>[4x]KRKIIFLSSPYGFSQQQKTLLLPPIVRALEALGIEVWEPFARNNQIDFSQADWAYRVAQADLQDVKNCDGIFAVVNGTPPDEGVMVELGMAIALNKAIFLFRDDFRRCSDNERYPLNLMLFAGLPEIGWENYYYTSVDEIQSHDKALYKWLTGM

Guided by the structure of the enzyme from the thermophilic organism Chroococcidiopsis thermalis PCC 7203 (CtNDT) bound to the ribonucleoside analogue Immucillin-H, we designed mutants of CtNDT and the psychrotolerant Bacillus psychrosaccharolyticus (BpNDT) to improve catalytic efficiency with 3′-deoxynucleosides and ribonucleosides, while maintaining nucleobase promiscuity to generate over 100 distinct nucleoside products. CtNDT has a preference for purine-based 2′-deoxynucleosides, while BpNDT prefers pyrimidine-based 2′-deoxynucleosides. Importantly, wild type CtNDT can utilize ribonucleoside and 3′-deoxynucleoside substrates, albeit with lower efficiency, demonstrating less strict selection of 2′-deoxynucleosides, and a possible strategy to produce 3′-deoxynucleosides. , As proof of concept, we determined cordycepin (3′-deoxyadenosine), a natural product currently employed to treat various types of cancers, can be used as a substrate by CtNDT. We have previously shown that this tyrosine residue in CtNDT (Y7) does not directly interact with the 2′-OH group, and instead positions the catalytic E88 for reaction.

We also determined the structure of a double mutant with improved catalytic efficiency toward 3′-deoxynucleosides and ribonucleosides, establishing a path to guide future NDT engineering which relies on modulating steric effects and electrostatics surrounding a conserved and essential catalytic glutamate residue. Our rationale was centered in (i) opening up the substrate binding pocket by mutating P40 and Y7 and (ii) and exploring additional hydrogen bonding interactions to better position a 2′-OH group by mutating A9 and V85. Figure c shows the complex structures of CtNDTY7F‑A9S and Cordycepin. A potential additional interaction between S9 and the catalytic E88 (distance 2.5 Å) is formed. This could be important to compensate for the loss in positioning previously conferred by Y7, mutated to a phenylalanine in this variant. In agreement with this, CtNDTY7F‑A9S showed an improvement on k cat/K M‑inosine of 8-fold in comparison to wild type, and a 2-fold improvement toward CtNDTY7F. The K D for Immucillin-H for the double mutant CtNDTY7F‑A9S is 590 μM, 7.5 times higher than the one determined for the wild-type protein, and close to the K M for inosine (620 μM), therefore binding in a substrate-like manner. On the top the overall tetramer is shown, and in the bottom a zoomed-in image of the substrate (cordycepin, dark blue) and mutated residues (marine blue), depicted here from CtNDTY7F‑A9S. We established a workflow to determine optimal reaction conditions and generated a mutant (CtNDTY7F‑A9S) with altered nucleoside substrate specificity toward 3′-deoxynucleosides and ribonucleoside substrates.> HHHHHHDFHVEEELDWPGVYLLPGQVSGVALDSKNNLVIFHRGDHVWDGNSFDSKFV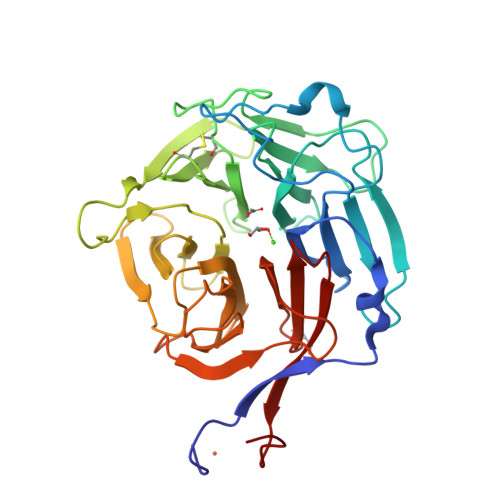YQQRGLGPIEEDTILVIDPNNAEILQSSGKNLFYLPHGLSIDTDGNYWVTDVALHQVFKLDPHSKEGPLLILGRSMQPGSDQNHFCQPTDVAVEPSTGAVFVSDGYCNSRIVQFSPSGKFVTQWGEESSGSSPRPGQFSVPHSLALVPHLDQLCVADRENGRIQCFKTDTKEFVREIKHASFGRNVFAISYIPGFLFAVNGKPYFGDQEPVQGFVMNFSSGEIIDVFKPVRKHFDMPHDIVASEDGTVYIGDAHTNTVWKFTLTEKMEHRSV>[2x]MHSFASLLAYGLVAGATFASASPIEARDSCTFTTAAAAKAGKAKCSTITLNNIEVPAGTTLDLTGLTSGTKVIFEGTTTFQYEEWAGPLISMSGEHITVTGASGHLINCDGARWWDGKGTSGKKKPKFFYAHGLDSSSITGLNIK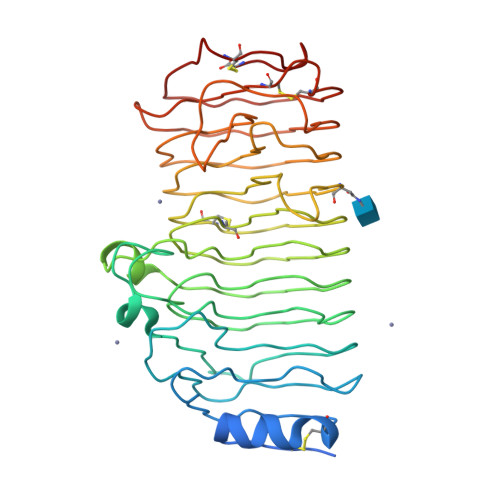NTPLMAFSVQANDITFTDVTINNADGDTQGGHNTDAFDVGNSVGVNIIKPWVHNQDDCLAVNSGENIWFTGGTCIGGHGLSIGSVGDRSNNVVKNVTIEHSTVSNSENAVRIKTISGATGSVSEITYSNIVMSGISDYGVVIQQDYEDGKPTGKPTNGVTIQDVKLESVTGSVDSGATEIYLLCGSGSCSDWTWDDVKVTGGKKSTACKNFPSVASC>EVDCELQPVIEANLSLNQNQLASNGGYISSQLGIRNESCETVKFKYWLSIKGPEGIYFPAKAVVGVDTAQQESDALTDGRMLNVTRGFWVPEYMADGKYTVSLQVVAENGKVFKANQEFVKGVDLNSLPELNGLTIDIKNQFGINSVESTGGFVPFTVDLNNGREGEANVEFWMTAVGPDGLIIPVNAREKWVIASGDTYSKVRGINFDKSYPAGEYTINAQVVDIVSGERVEQSMTVVKK[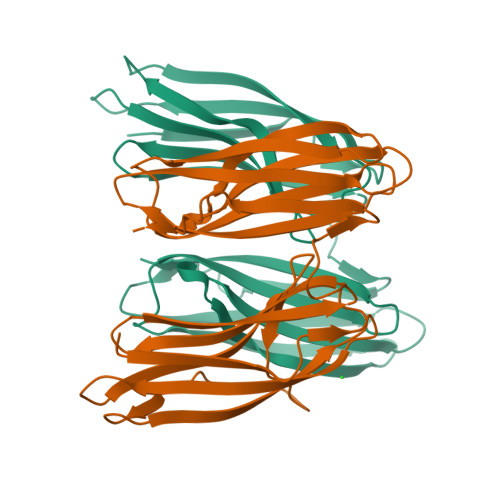2x]>[2x]SNAMELEQKLNLLNDLIVREIVNPLPPPYKVGVDLGTADIVLVVTDQEGIPVAGALKWASVVKDGL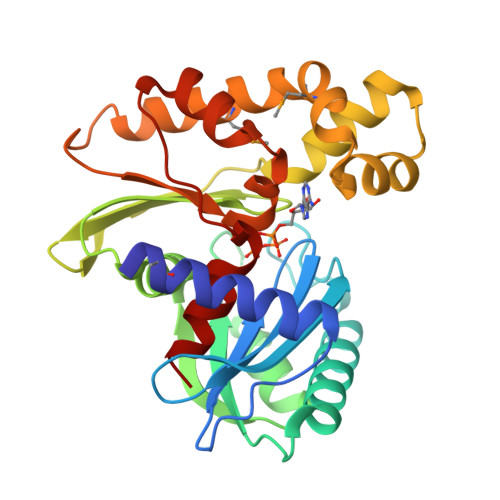VVDYIGAIQIVRELKAKVERLLGSELFQAATAIPPGTVGRNAEACGHVVAGAGLELVTLVDEPVAAARALGINDGIVVDIGGGTTGIAVIEKGKITATFDEPTGGTHLSLVLAGSYKIPFEEAETIKKDFSRHREIMRVVRPVIEKMALIVKEVIKNYDQTLPVYVVGGTAYLTGFSEEFSRFLGKEVQVPIHPLLVTPLGIALFG GLYCYL-ADENOSINE-5'-PHOSPHATE 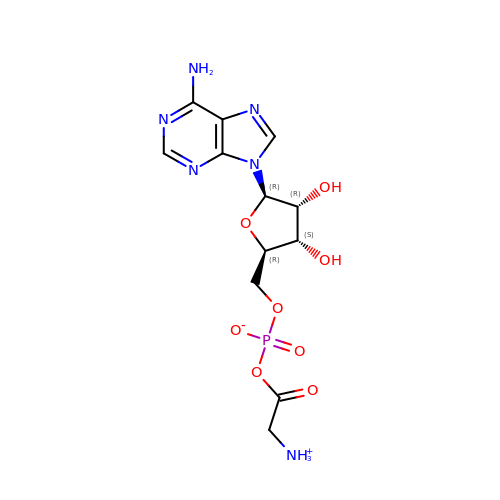| C12 H17 N6 O8 P | HROXHMRQKGGIFT-JJNLEZRASA-N1,3-dihydroxypropan-2-yl butanoate | C7 H14 O4 | 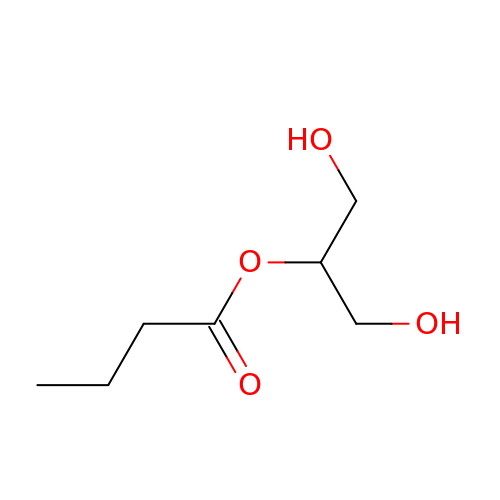PVPWPCLNZDBNFK-UHFFFAOYSA-N> QGEFMEPRAVADALETGEEDAVTEALRSFNREHSQSFTFDDAQQEDRKRLAKLLVSVLEQGLSPKHRVTWLQTIRILSRDRSCLDSFASRQSLHALACYADIAISEEPIPQPPDMDVLLESLKCLCNLVLSSPTAQMLAAEARLVVRLAERVGLYRKRSYPHEVQFFDLRLLFLLTALRTDVRQQLFQELHGVRLLTDALELTLGVAPKENPLVILPAQETER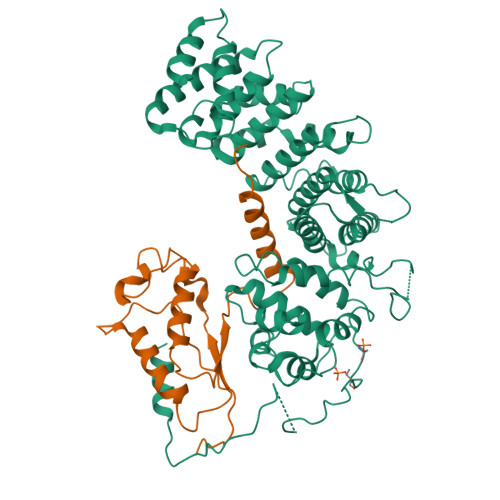AMEILKVLFNITFDSVKREVDEEDAALYRYLGTLLRHCVMADAAGDRTEEFHGHTVNLLGNLPLKCLDVLLALELHEGSLEFMGVNMDVINALLAFLEKRLHQTHRLKECVAPVLSVLTECARMHRPARKFLKAQVLPPLRDVRTRPEVGDLLRNKLVRLMTHLDTDVKRVAAEFLFVLCSESVPRFIKYTGYGNAAGLLAARGLMAGGRPEGQYSEDEDTDTEEYREAKASXXXXXXXXXXXXXXXXXXXXXXXXXXX;> MTLESIMACCLSEEAKEARRINDEIERQLRRDKRDARRELKLLLLGTGESGKSTFIKQMRIIHGSGYSDEDKRGFTKLVYQNIFTAMQAMIRAMDTLKIPYKYEHNKAHAQLVREVDVEKVSAFENPYVDAIKSLWNDPGIQECYDRRREYQLSDSTKYYLNDLDRVADPAYLPTQQDVLRVRVPTTGIIEYPFDLQSVIFRMVDVGGQRSERRKWIHCFENVTSIMFLVALSEYDQVLVESDNENRMEESKALFRTIITYPWFQNSSVILFLNKKDLLEEKIMYSHLVDYFPEYDGPQRDAQAAREFILKMFVDLNPDSDKIIYSHFTCATDTENIRFVFAAVKDTILQLNLKEYNLV>[6x]GSSERPSPPVNLTSSDQTQSSVQLKWEPP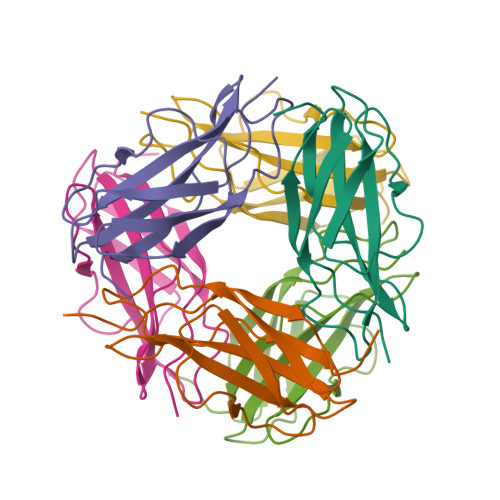LKDGGSPILGYIIERCEEGKDNWIHCNMKLVPELTYKVTGLEKGNKYLYRVSAENKAGVSDPSEILGPLTADDAFVE>VIPVEEENPVFWNQKAKEALDVAKKLQPIQTSAKNLILFLGDGMGVPTVTATRILKGQLGGHLGPETPLAMDHFPFTALSKTYNVDRQVPDSAGTATAYLCGVKANYKTIGVSAAARFNQCNSTFGNEVFSVMHRAKKAGKSVGVVTTTRVQHASPAGTYAHTVNRDWYSDADMPSSALQEGCKDIATQLISNMDIDVILGGGRKFMFPKGTPDPEYPGDSDQSGVRLDSRNLVEEWLAKYQGTRYVWNREQLMQASQDPAVTRLMGLFEPTEMKYDVNRNASADPSLAEMTEVAVRLLSRNPQGFYLFVEGGRIDQGHHAGTAYLALTEAVMFDSAIEKASQLTNEKDTLTLITADHSHVFAFGGYTLRGTSIFGLAPLNAQDGKSYTSILYGNGPGYVLNSGNRPNVTDAESGDVNYKQQAAVPLSSETHGGEDVAIFARGPQAHLVHGVQEQNYIAHVMA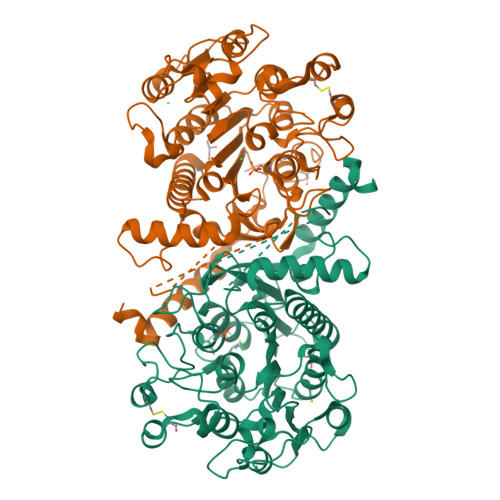FAGCLEPYTDCGLAPPADEHHHHHH[2x]>MKKLGTLLVLFLSAIILVACASGKKDTTSGQKLKVVATNSIIADITKNIAGDKIDLHSIVPIGQDPHEYEPLPEDVKKTSEADLIFYNGINLETGGNAWFTKLVENAKKTENKDYFAVSDGVDVIYLEGQNEKGKEDPHAWLNLENGIIFAKNIAKQLSAKDPNNKEFYEKNLKEYTDKLDKLDKESKDKFNKIPAEKKLIVTSEGAFKYFSKAYGVPSAYIWEINTEEEGTPEQIKTLVEKLRQTKVPSLFVESSVDDRPMKTVSQDTNIPIYAQIFTNSIAEQGKEGDSYYSMMKYNLDKIAEGLAK[2x]

The pneumococcus acquires Mn2+ via the PsaBCA permease, which comprises the ATP-binding cassette (ABC) transporter, PsaBC, and a cell-surface solute-binding protein (SBP), PsaA. Similar to other ABC permeases, the SBP PsaA defines the specificity of the uptake pathway. However, our recent studies showed that the functional specificity of the Psa permease in Mn2+ acquisition arose not from the specificity of Mn2+ binding by PsaA, but instead resulted from the concerted action of protein metal ion coordination chemistry and structural rearrangements that prevented release of other divalent transition metal ions, such as Zn2+, into the permease, despite their ability to bind to PsaA8. PsaA uses a ‘spring-hammer’-like mechanism for metal ion binding, in which the dynamics of the metal ion-loaded protein are dictated by a combination of metal ion geometry and the distortion of a helix linking the N- and C-terminal lobes of the protein.

We further analysed the metal-binding site coordination geometry by use of an Asp280 variant isoform (PsaA-D280N), as it would be incapable of facilitating the trigonal-bipyramidal coordination observed in wild-type PsaA8. The structure of PsaA-D280N bound to Cd2+, refined to 1.7 Å resolution, revealed a partially solvated Cd ion loosely interacting with residue Glu205. The C-terminal lobe of PsaA showed minor movement (~1.0° relative to the open, metal-free conformation), but the inability of Cd2+ to ligate to residue Asp280 prevented further conformational changes. Consistent with these observations, PsaA-D280N was greatly impaired in Cd2+ binding.> MHHHHHHAQTLNSYKMAEIMYKILEKKGELTLEDILAQFEISVPSAY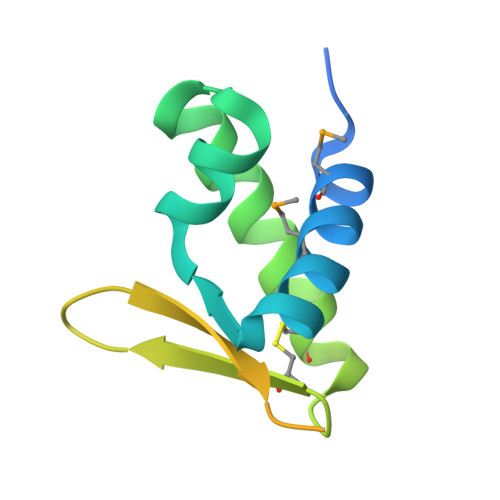NIQRALKAICERHPDECEVQYKNRKTTFKWIKQEQKEEQKQEQTQDNIAKIFDAQPANFEQTDQGFIKAKQ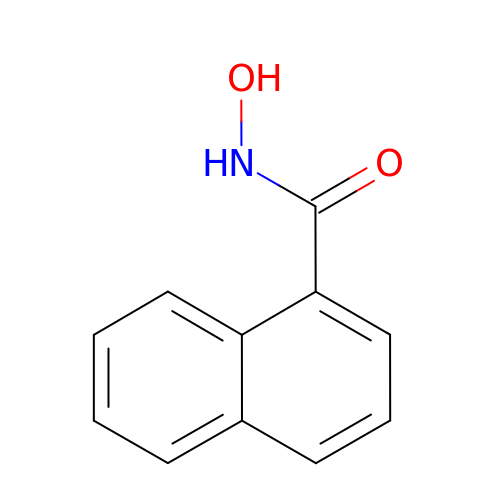~{N}-oxidanylnaphthalene-1-carboxamide | C11 H9 N O2 | JRZGPWOEHDOVMC-UHFFFAOYSA-N>MEDLSSLTPGGSMGLQVNRGSQSSLEGAPATAPEPHSLGILHASYSVSHRVRPWWDITSCRQQWTRQILKDVSLYVESGQIMCILGSSGSGKTTLLDAMSGRLGRAGTFLGEVYVNGRALRREQFQDCFSYVLQSDTLLSSLTVRETLHYTALLAIRRGNPGSFQKKVEAVMAELSLSHVADRLIGNYSLGGISTGERRRVSIAAQLLQDPKVMLFDEPTTGLDCMTANQIVVLLVELARRNRIVVLTIHQPRSELFQLFDKIAILSFGELIFCGTPAEMLDFFNDCGYPCPEHSNPFDFYMDLTSVDTQSKEREIETSKRVQMIESAYKKSAICHKTLKNIERMKHLKTLPMVPFKTKDSPGVFSKLGVLLRRVTRNLVRNKLAVITRLLQNLIMGLFLLFFVLRVRSNVLKGAIQDRVGLLYQFVGATPYTGMLNAVNLFPVLRAVSDQESQDGLYQKWQMMLAYALHVLPFSVVATMIFSSVCYWTLGLHPEVARFGYFSAALLAPHLIGEFLTLVLLGIVQNPNIVNSVVALLSIAGVLVGSGFLRNIQEMPIPFKIISYFTFQKYCSEILVVNEFYGLNFTCGSSNVSVTTNPMCAFTQGIQFIEKTCPGATSRFTMNFLILYSFIPALVILGIVVFKIRDHLISRGSHHHHHHGHHHHHH[2x];>[2x]MGSAGKAAEERGLPKGATPQDTSGLQDRLFSSESDNSLYFTYSGQPNTLEVRDLNYQVDLASQVPWFEQLAQFKMPWTSPSCQNSCELGIQNLSFKVRSGQMLAIIGSSGCGRASLLDVITGRGHGGKIKSGQIWINGQPSSPQLVRKCVAHVRQHNQLLPNLTVRETLAFIAQMRLPRTFSQAQRDKRVEDVIAELRLRQCADTRVGNMYVRGLSGGERRRVSIGVQLLWNPGILILDEPTSGLDSFTAHNLVKTLSRLAKGNRLVLISLHQPRSDIFRLFDLVLLMTSGTPIYLGAAQHMVQYFTAIGYPCPRYSNPADFYVDLTSIDRRSREQELATREKAQSLAALFLEKVRDLDDFLWKAETKDLDEDTCVESSVTPLDTNCLPSPTKMPGAVQQFTTLIRRQISNDFRDLPTLLIHGAEACLMSMTIGFLYFGHGSIQLSFMDTAALLFMIGALIPFNVILDVISKCYSERAMLYYELEDGLYTTGPYFFAKILGELPEHCAYIIIYGMPTYWLANLR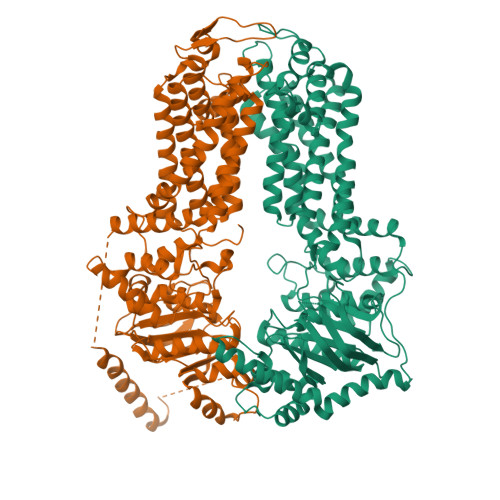PGLQPFLLHFLLVWLVVFCCRIMALAAAALLPTFHMASFFSNALYNSFYLAGGFMINLSSLWTVPAWISKVSFLRWCFEGLMKIQFSRRTYKMPLGNLTIAVSGDKILSVMELDSYPLYAIYLIVIGLSGGFMVLYYVSLRFIKQKPSQDWASNSLEVLFQ> MGSSHHHHHHSSGTAEPEVRAKPYTLEEFSYDYFRPPPKHTLSRVMVSKARGKDRLWSHTREPLKQALLKKLL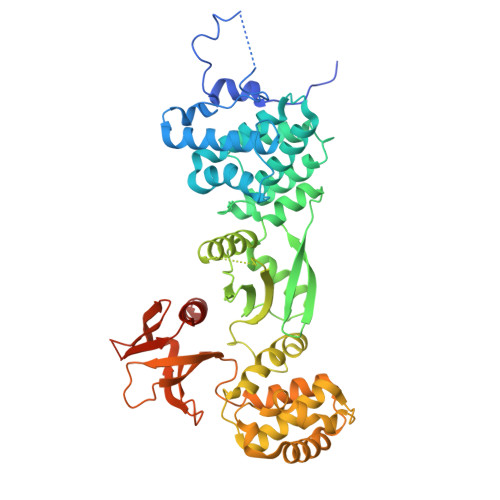GSEELSQEACLAFIAVLKYMGDYPSKRTRSVNELTDQIFEGPLKAEPLKDEAYVQILKQLTDNHIRYSEERGWELLWLCTGLFPPSNILLPHVQRFLQSRKHCPLAIDCLQRLQKALRNGSRKYPPHLVEVEAIQHKTTQIFHKVYFPDDTDEAFEVESSTKAKDFCQNIATRLLLKSSEGFSLFVKIADKVLSVPENDFFFDFVRHLTDWIKKARPIKDGIVPSLTYQVFFMKKLWTTTVPGKDPMADSIFHYYQELPKYLRGYHKCTREEVLQLGALIYRVKFEEDKSYFPSIPKLLRELVPQDLIRQVSPDDWKRSIVAYFNKHAGKSKEEAKLAFLKLIFKWPTFGSAFFEVKQTTEPNFPEILLIAINKYGVSLIDPKTKDILTTHPFTKISNWSSGNTYFHITIGNLVRGSKLLCETSLGYKMDDLLTSYISQMLTAMSKQRGSRSGK>[2x]GAMGSGGISEEEAAQYDRQIRLWGLEAQKRLRASRVLLVGLKGLGAEIAKNLILAGVKGLTMLDHEQVTPEDPGAQFLIRTGSV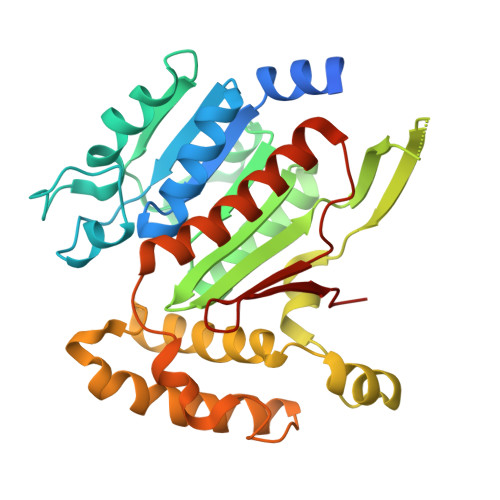GRNRAEASLERAQNLNPMVDVKVDTEDIEKKPESFFTQFDAVCLTCCSRDVIVKVDQICHKNSIKFFTGDVFGYHGYTFANLGEHEFVEEKTETTMVKKKVVFCPVKEALEVDWSSEKAKAALKRTTSDYFLLQVLLKFRTDKGRDPSSDTYEEDSELLLQIRNDVLDSLGISPDLLPEDFVRYCFSEMAPVCAVVGGILAQEIVKALSQRDPPHNNFFFFDGMKGNGIVECLGPK>[4x]GFPLITITVRGRNVHMKQEHYMKGSDGAPDTGYLWHVPLTFITSKSDMVHRFLLKTKTDVLILPEEVEWIKFNVGMNGYYIVHYEDDGWDSLTGLLKGTHTAVSSNDRASLINNAFQLVSIGKLSIEK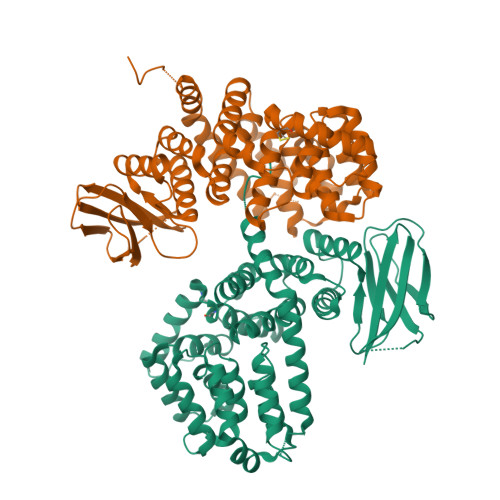ALDLSLYLKHETEIMPVFQGLNELIPMYKLMEKRDMNEVETQFKAFLIRLLRDLIDKQTWTDEGSVSERMLRSQLLLLACVHNYQPCVQRAEGYFRKWKESNGNLSLPVDVTLAVFAVGAQSTEGWDFLYSKYQFSLSSTEKSQIEFALCRTQNKEKLQWLLDESFKGDKIKTQEFPQILTLIGRNPVGYPLAWQFLRKNWNKLVQKFELGSSSIAHMVMGTTNQFSTRTRLEEVKGFFSSLKENGSQLRCVQQTIETIEENIGWMDKNFDKIRVWLQSEKLERMFKARKF> MVLFSTYRSSRLVSKEFLHGPVMRFRALGEYYFQRAWNGTLNWALPGEYRLYAVMIPFIYFYHRWHNDHT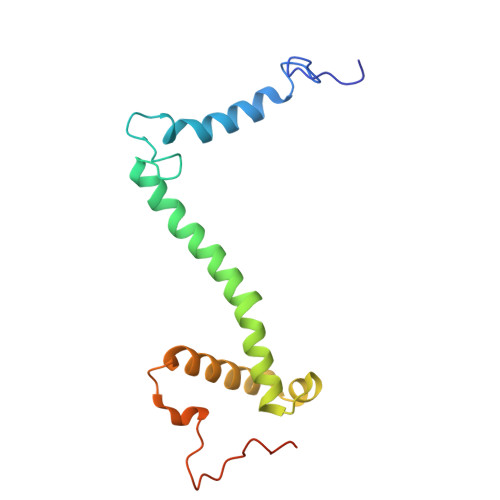LDRDHVEKAMIMRWGGTLEDVRKLSAKDQLRVRCFTDIEKLYSAYGPKDTYLQPPGDTLPGKDFYRKAGGAQAHH>[4x]PPRKVLIISAGA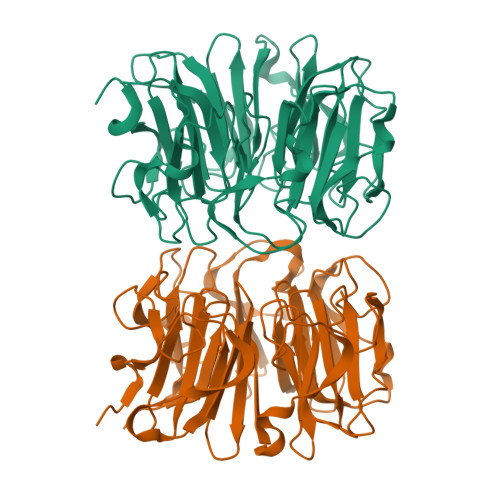SHSVALLSGDIVCSWGRGEDGQLGHGDAEDRPSPTQLSALDGHQIVSVTCGADHTVAYSQSGMEVYSWGWGDFGRLGHGNSSDLFTPLPIKALHGIRIKQIACGDSHCLAVTMEGEVQSWGRNQNGQLGLGDTEDSLVPQKIQAFEGIRIKMVAAGAEHTAAVTEDGDLYGWGWGRYGNLGLGDRTDRLVPERVTSTGGEKMSMVACGWRHTISVSYSGALYTYGWSKYGQLGHGDLEDHLIPHKLEALSNSFISQISGGWRHTMALTSDGKLYGWGWNKFGQVGVGNNLDQCSPVQVRFPDDQKVVQVSCGWRHTLAVTERNNVFAWGRGTNGQLGIGESVDRNFPKIIEALSVDGLEHHHHHH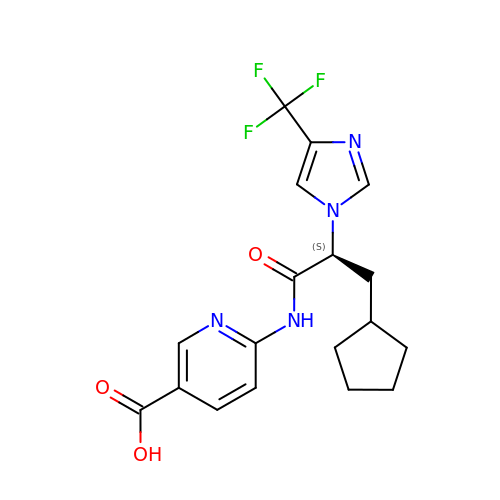6-({(2S)-3-cyclopentyl-2-[4-(trifluoromethyl)-1H-imidazol-1-yl]propanoyl}amino)pyridine-3-carboxylic acid | C18 H19 F3 N4 O3 | GKMLFBRLRVQVJO-ZDUSSCGKSA-N>[2x]MASWSHPQFEKGADDDDKVPDPTSVDSVKYSKIKGIPKLDDANDAGGKHSLECTLILTEGDSAKSLAVSGLGVIGRDRYGVFPLRGKILNVREASHKQIMENAEINNIIKIVGLQYKKSYDDAESLKTLRYGKIMIMTDQDQDGSHIKGLLINFIHHNWPSLLKHGFLEEFITPIVKASKNKQELSFYSIPEFDEWKKHIENQKAWKIKYYKGLGTSTAKEAKEYFADMERHRILFRYAGPEDDAAITLAFSKKKIDDRKEWLTNFMEDRRQRRLHGLPEQFLYGTATKHLTYNDFINKELILFSNSDNERSIPSLVDGFKPGQRKVLFTCFKRNDKREVKVAQLAGSVAEMSAYHHGEQALMMTIVNLAQNFVGSNNINLLQPIGQFGTRLHGGKDAASPRYIFTMLSTLARLLFPAVDDNLLKFLYDDNQRVEPEWYIPIIPMVLINGAEGIGTGWACKLPNYDAREIVNNVRRMLDGLDPHPMLPNYKNFKGTIQELGQNQYAVSGEIFVVDRNTVEITELPVRTWTQVYKEQVLEPMLNGTDKTPALISDYKEYHTDTTVKFVVKMTEEKLAQAEAAGLHKVFKLQTTLTCNSMVLFDHMGCLKKYETVQDILKEFFDLRLSYYGLRKEWLVGMLGAESTKLNNQARFILEKIQGKITIENRSKKDLIQMLVQRGYESDPVKAWKEAQEKAAEEDETQNQHDDSSSDSGTPSGPDFNYILNMSLWSLTKEKVEELIKQRDAKGREVNDLKRKSPSDLWKEDLAAFVEELDKVESQEREDGAPGFSSISAHHHHHHHHHH

Type IIA topoisomerases (Top2s) are essential DNA-manipulating enzymes ubiquitous in eukaryotes and bacteria. These enzymes exploit protein conformational changes driven by ATP binding and hydrolysis to direct the crossing of two DNA duplexes, leading to topological inversion of DNA crossovers. The Top2-mediated DNA topological transformation requires the temporary creation of a DNA double-strand break (DSB) on one DNA segment (the G-segment), so that another duplex strand (the T-segment) can be transported through.

Because iodine is substantially more electron-rich than the 5-methyl group of thymine, the use of 5-iodouridine allowed the positions of thymine nucleotides to be unambiguously recognized in the difference electron density map. However, if the G-segment DNA is cleaved as intended, then the I-labels should appear on the +1, +7, and +12 locations in one of the complementary strands in each half of the DNA-gate. This expectation is validated by our observation that the difference peaks in the previously solved closed conformation of the Top2 cleavage complex are nicely overlaid with C5-methyl groups of the three thymidine residues. Crystallographic studies have revealed that these drugs interact with the closed conformation of the DNA-gate and inhibit the religation of cleaved G-segment by inserting into the DNA cleavage sites.> HNHNHNHNHNHNGGENLYFQGASLTEIEHLVQSVCKSY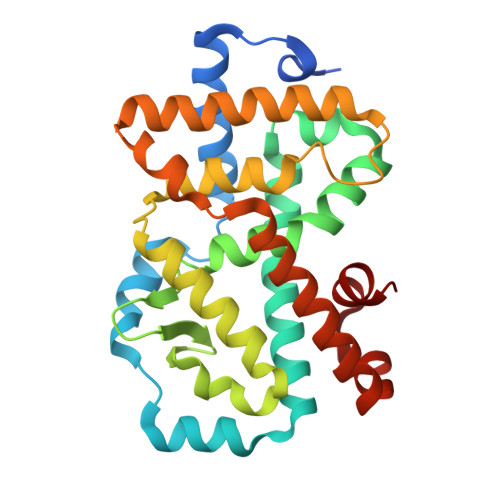RETCQLRLEDLLRQRSNIFSREEVTGYQRKSMWEMWERCAHHLTEAIQYVVEFAKRLSGFMELCQNDQIVLLKAGAMEVVLVRMCRAYNADNRTVFFEGKYGGMELFRALGCSELISSIFDFSHSLSALHFSEDEIALYTALVLINAHRPGLQEKRKVEQLQYNLELAFHHHLCKTHRQSILAKLPPKGKLRSLCSQHVERLQIFQHLHPIVVQAAFPPLYKELFSGG> QPIFLNVLEAIEPGVVCAGHDNNQPDSFAALLSSLNELGERQLVHVVKWAKALPGFRNLHVDDQMAVIQYSWMGLMVFAMGWRSFTNVNSRMLYFAPDLVFNEYRMHKSRMYSQCVRMRHLSQEFGWLQITPQEFLCMKALLLFSIIPVDGLKNQKFFDELRMNYIKELDRIIACKRKNPTSCSRRFYQLTKLLDSV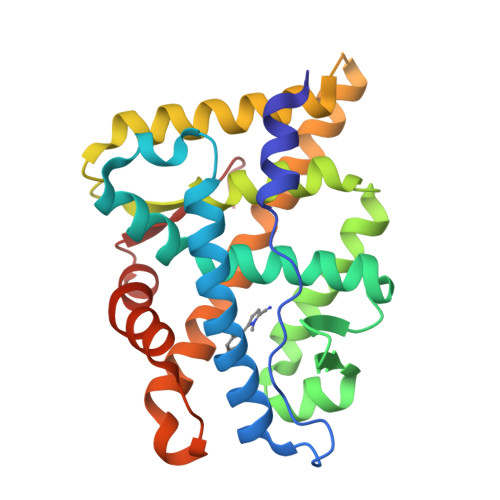QPIARELHQFTFDLLIKSHMVSVDFPEMMAEIISVQVPKILSGKVKPIYFHTQ>MKTIFSGIQPSGVITIGNYIGALRQFVELQHEYNCYFCIVDQHAITVWQDPHELRQNIRRLAALYLAVGIDPTQATLFIQSEVPAHAQAAWMLQCIVYIGELERMTQFKEKSAGKEAVSAGLLTYPPLMAADILLYNTDIVPVGEDQKQHIELTRDLAERFNKRYGELFTIPEARIPKVGARIMSLVDPTKKMSKSDPNPKAYITLLDDAKTIEKKIKSAVTDSEGTIRYDKEAKPGISNLLNIYSTLSGQSIEELERQYEGKGYGVFKADLAQVVIETLRPIQERYHHWMESEELDRVLDEGAEKA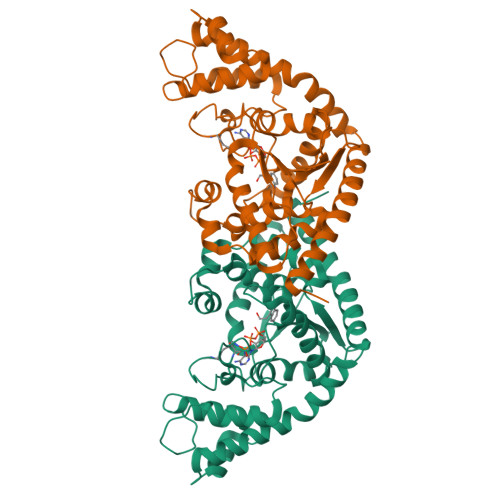NRVASEMVRKMEQAMGLGRRRLE[4x]2-BROMO-6-CHLORO-PURINE | C5 H2 Br Cl N4 | 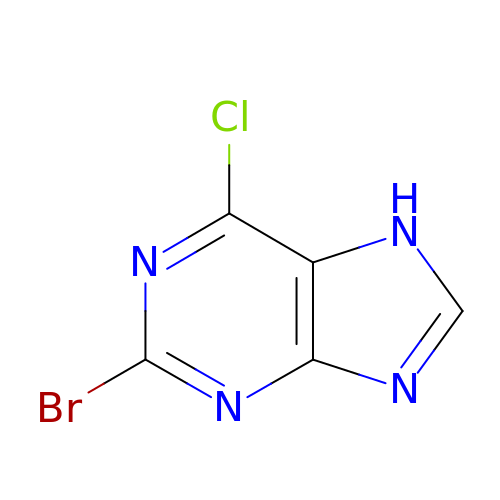VLGHYTLGJNPTEN-UHFFFAOYSA-N> IVGGQECKDGECPWQALLINEENEGFCGGTILSEFYILTAAHCLYQAKRFKVRVGDRNTEQEEGGEAVHEVEVVIKHNRFTKETYDFDIAVLRLKTPITFRMNVAPACLPERDWAESTLMTQKTGIVSGFGRTHEKGRQSTRLKMLEVPYVDRNSCKLSSSFIITQNMFCAGYDTKQEDACQGDSGGPHVTRFKDTYFVTGIVSWGEGCARKGKYGIYTKVTAFLKWIDRSMKTR;> DGDQC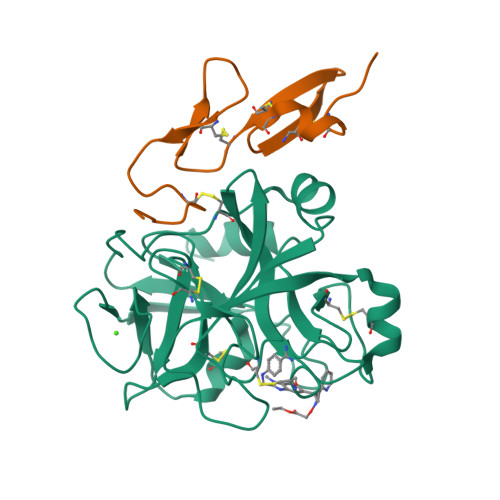ETSPCQNQGKCKDGLGEYTCTCLEGFEGKNCELFTRKLCSLDNGDCDQFCHEEQNSVVCSCARGYTLADNGKACIPTGPYPCGKQTLER>MLSRKGIIPEEYVLTRLAEDPAEPRYRTRERRARFVSKKGNCNVAHKNIREQGRFLQDVFTTLVDLKWPHTLLIFTMSFLCSWLLFAMVWWLIAFAHGDLAPGEGTNVPCVTSIHSFSSAFLFSIEVQVTIGFGGRMVTEECPLAILILIVQNIVGLMINAIMLGCIFMKTAQAKRRAETLIFSKHAVITLRHGRLCFMLRVGDLRKSMIISATIHMQVVRKTTSPEGEVVPLHQVDIPMENGVGGNGIFLVAPLIIYHVIDSNSPLYDLAPSDLHHHQDLEIIVILEGVVETTGITTQARTSYLADEILWGQRFVPIVAEEDGRYSVDYSKFGNTIKVPTPLCTARQLDEDRSLLDALTLASSRGPLRKRSVAVAKAKPKFSISPDSLS[4x];>[4x]MPLAFCGTENHSAAYRVDQGVLNNGCFVDALNVVPHVFLLFITFPILFIGWGSQSSKVHIHHSTWLHFPGHNLRWILTFILLFVLVCEIAEGILSDGVTESRHLHLYMPAGMAFMAAITSVVYYHNIETSNFPKLLIALLIYWTLAFITKTIKFVKFYDHAIGFSQLRFCLTGLLVILYGMLLLVEVNVIRVRRYIFFKTPREVKPPEDLQDLGVRFLQPFVNLLSKGTYWWMNAFIKTAHKKPIDLRAIGKLPIAMRALTNYQRLCVAFDAQARKDTQSPQGARAIWRALCHAFGRRLILSSTFRILADLLGFAGPLCIFGIVDHLGKENHVFQPKTQFLGVYFVSSQEFLGNAYVLAVLLFLALLLQRTFLQASYYVAIETGINLRGAIQTKIYNKIMHLSTSNLSMGEMTAGQICNLVAIDTNQLMWFFFLCPNLWAMPVQIIVGVILLYYILGVSALIGAAVIILLAPVQYFVATKLSQAQRSTLEHSNERLKQTNEMLRGMKLLKLYAWESIFCSRVEVTRRKEMTSLRAFAVYTSISIFMNTAIPIAAVLITFVGHVSFFKESDLSPSVAFASLSLFHILVTPLFLLSSVVRSTVKALVSVQKLSEFLSSAEIREEQCAPREPAPQGQAGKYQAVPLKVVNRKRPAREEVRDLLGPLQRLAPSMDGDADNFCVQIIGGFFTWTPDGIPTLSNITIRIPRGQLTMIVGQVGCGKSSLLLATLGEMQKVSGAVFWNSNLPDSEGEDPSSPERETAAGSDIRSRGPVAYASQKPWLLNATVEENITFESPFNKQRYKMVIEACSLQPDIDILPHGDQTQIGERGINLSGGQRQRISVARALYQQTNVVFLDDPFSALDVHLSDHLMQAGILELLRDDKRTVVLVTHKLQYLPHADWIIAMKDGTIQREGTLKDFQRSECQLFEHWKTLMNRQDQELEKETVMERKASEPSQGLPRAMSSRDGLLLDEEEEEEEAAESEEDDNLSSVLHQRAKIPWRACTKYLSSAGILLLSLLVFSQLLKHMVLVAIDYWLAKWTDSALVLSPAARNCSLSQECDLDQSVYAMVFTLLCSLGIVLCLVTSVTVEWTGLKVAKRLHRSLLNRIILAPMRFFETTPLGSILNRFSSDCNTIDQHIPSTLECLSRSTLLCVSALTVISYVTPVFLVALLPLAVVCYFIQKYFRVASRDLQQLDDTTQLPLLSHFAETVEGLTTIRAFRYEARFQQKLLEYTDSNNIASLFLTAANRWLEVRMEYIGACVVLIAAATSISNSLHRELSAGLVGLGLTYALMVSNYLNWMVRNLADMEIQLGAVKRIHALLKTEAESYEGLLAPSLIPKNWPDQGKIQIQNLSVRYDSSLKPVLKHVNALISPGQKIGICGRTGSGKSSFSLAFFRMVDMFEGRIIIDGIDIAKLPLHTLRSRLSIILQDPVLFSGTIRFNLDPEKKCSDSTLWEALEIAQLKLVVKALPGGLDAIITEGGENFSQGQRQLFCLARAFVRKTSIFIMDEATASIDMATENILQKVVMTAFADRTVVTIAHRVHTILSADLVMVLKRGAILEFDKPETLLSQKDSVFASFVRADK

ATP-sensitive potassium channels (KATP) are metabolic sensors that convert the intracellular ATP/ADP ratio to the excitability of cells. Functional KATP channels are hetero-octamers composed of four Kir6 and four SUR subunits. Kir6 are inward rectifier potassium channels that require PI(4,5)P2 for maximum activity. The SUR subunits bind to activating Mg-ADP and drugs, including insulin secretagogues and KATP openers.

Based on these observations, we made H175K mutation on the SUR1-Kir6.2 fusion constructs, in which the C terminus of SUR1 is covalently linked to the N terminus of Kir6.2 by a long linker to ensure the correct 4:4 stoichiometry between Kir6.2 and SUR126, yielding the H175Kcryo-EM construct. Subsequent refinement resolved two 3D classes: one class has a closed and the other has a widened inner helix gate. In contrast, in the structure with widened gate, the inner part of the M2 helix moves outward. Particularly, the side chains of L164 and F168 move away from the center, resulting in the dilation of the pore. The radius of the ion permeation pathway at the bundle crossing of TMD now increases to 3 Å. However, the constriction at the cytosolic G-loop gate still shows a radius of 2.6 Å. While in the pre-open state, the side chains of F60 swing away, which allows the expansion of M2. In contrast, there is no ADP density in the pre-open state, and we observed an obvious structural reorganization around the nucleotide-binding pocket of Kir6.2. During channel opening, there is a 6° anti-clockwise rotation of CTD viewing from the intracellular side, resulting in the clash between E51 and the nucleotide-binding pocket in the pre-open state. Although the ion permeation pathway of the pre-open state does not allow the permeation of fully hydrated potassium ions, the hallmarks of KATP channel activation, such as the enlargement of inner helix gate of Kir6.2, the dissociation of inhibitory nucleotide from Kir6.2, the rotation of Kir6.2 CTD, and the binding of activator NN414 and activatory Mg-nucleotides on NBD-dimerized SUR1, all suggest the current pre-open structure represents the “activated” state of KATP.> MEHYSTIQNSLNDKIVTISCKANTDLFFYQVPGNGNVSLFQQTRNYLERWRIIYDSNKAAYKIKSMNIYNTNLVLTWNAPTHNISAQQDSNADNQYWLLLKDIGNNSFIIASYKNPNLVLYADTVARNLKLSTLNNSSYIKFIIEDYVISDFKNFTCRISPILAG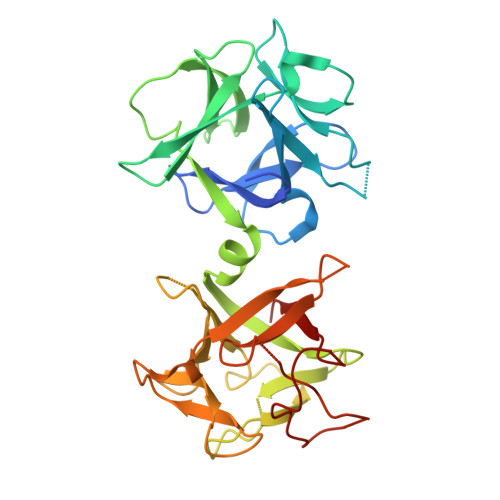GKVVQQVSMTNLAVNLYIWNNDLNQKWTIIYNEEKAAYQFFNKILSNGVLTWIFSDGNTVRVSSSAQNNDAQYWLINPVSDNYDRYTITNLRDKTKVLDLYGGQTADGTTIQVFNSNGGDNQIWTMSNP Inositol pyrophosphates (PP-InsPs) are eukaryotic nutrient messengers. The N-terminal kinase domain of diphosphoinositol pentakisphosphate kinase (PPIP5K) generates the messenger 1,5-InsP8, the C-terminal phosphatase domain catalyzes PP-InsP breakdown. The balance between kinase and phosphatase activities regulates 1,5-InsP8 levels. ScVip1PD is a phytase-like inositol 1-pyrophosphate histidine phosphatase with two conserved catalytic motifs.

Crystallization of ScVip1PD Δ848-918 yielded a second crystal form diffracting at 3.4 Å resolution. The two apo structures of ScVip1PD revealed a conserved histidine acid phosphatase core with two insertion domains. In ScVip1PD Δ848-918 crystals, two molecules in the asymmetric unit also adopt the “open” conformation. Crystal packing interactions between two adjacent GAF domains in our ScVip1PD Δ848-918 crystals are mediated in part by a second Zn2+ binding site. The Zn2+ ion is coordinated along a pseudo two-fold axis involving residues His573 and Glu575 from the GAF domain. Given that ScVip1PD behaves as a monomer in solution and that the histidine and glutamate residues are not conserved among other PPIP5Ks, the second Zn2+ coordination site is likely a crystallization artifact. Similarly, deletion of the large disordered loop in the α-helical insertion domain (ScVip1PD Δ848-918) moderately activates the engineered enzyme in vitro.

>[4x]GAKWVFKGLAIIIRHADRTPKQKFKHSFTSPIFISLLKGHKEEVVIRNVNDLKIVLQALRIALDEKAGNPAKIKVLANALEKKLNFPGTKIQLKPVLNKENEVEKVQFILKWGGEPTHSAKYQATELGEQMRQDFDLLNKSILQNIKIFSSSERRVLHTAQYWTRALFGADELGSDEISIRKDLLDDSNAAKDLMDKVKKKLKPLLREGKEAPPQFAWPSKMPEPYLVIKRVVELMNYHKKIMDNNFAKKDVNSMQTRWCTSEDPSLFKERWDKLFKEFNNAEKVDPSKISELYDTMKYDALHNRQFLENIFDPGSSGQFDEPRFMQLRELYKLAKVLFDFICPKEYGISDAEKLDIGLLTSLPLAKQILNDIGDMKNRETPACVAYFTKESHIYTLLNIIYESGIPMRIARNALPELDYLSQITFELYESTDASGQKSHSIRLKMSPGCHTQDPLDVQLDDRHYISCIPKISLTKHLDMDYVQQKLRNKFTRVIMPPKFTPVNITS> GSSMASANLEGDALHTLRVTLVDPNNVLQSWDPTLVNPCTWFHVTCNNENSVIRVDLGNAELSGHLVPELGVLKNLQYLELYSNNITGPIPSNLGNLTNLVSLDLYLNSFSGPIPESLGKLSKLRFLRLNNNSLTG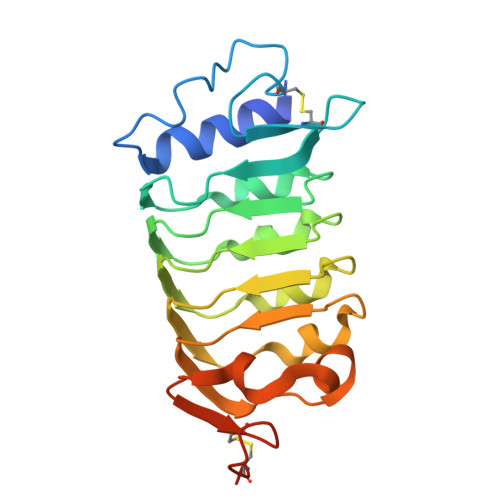SIPMSLTNITTLQVLDLSNNRLSGSVPDNGSFSLFTPISFANNLDLCGPVTSHPCPLEGSLENLYFQ> SFGSDVRPAAAQEVVGGGDLGPNVLVFDPSTPDIQGKVDEVFRKQESNQFGTDRYALMFKPGTYNDINAQIGFYTSIAGLGLNPDDTTFNGDVTVDAGWFDGNATQNFWRSAENLALNPVNGTNRWAVSQAAPFRRMHVKGGLNLAPDGYGWASGGYIADSKIDGEVGPYSQQQWYTRDSSVGGWGNGVWNMTFSGVEGAPAQSFPEPPYTTLETTPVSREKPFLYLDGDDYKVFVPAKRTNARGTSWGNGTPEGESLPLDQFYVVKPGATAETINAAVDQGLHLLFTPGVYHVDQPIEIDRANTVALGLGLATIIPDNGVTALKVGDVDGVKVAGLLVDAGPVNSETLVEVGSDGASGDHAANPTSLQDVFVRIGGAGPGKATTSIVVNSNDTIIDHTWVWRADHGEGVGWETNRADYGVHVKGDNV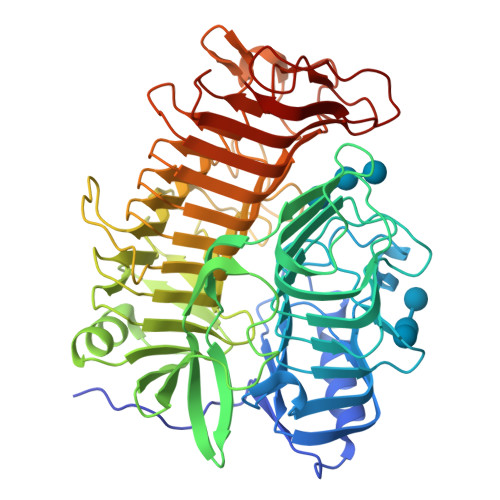LATGLFVEHFNKYDVQWSGENGKTIFYQNAKAYDAPDQAAIQNGDIKGYAAYKVDDSVTTHEGWGMGSYCYFNVNPDIRQQHGFQAPVKPGVKFHDLLVVSLGGKGQYEHVINDIGDPTSGDTTIPSQVVSFP> CUCUGUUUACCAGGUCAGGUCCGGAAGGAAGCAGCCAAG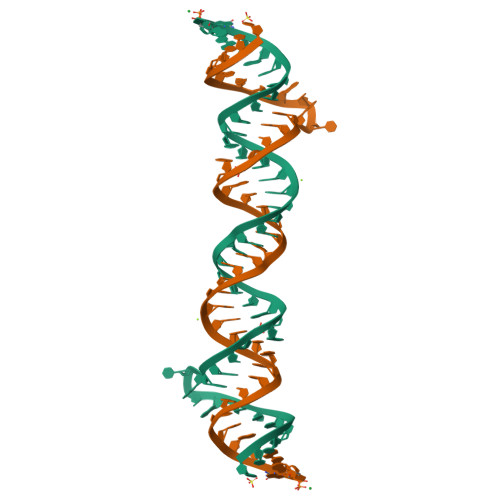GCAGAG>[8x]MGAGAGARWGSRAPEAPQPARAAGPGDVVVPCHGEHQAGIVTPPPSFIALVALDLASTSDRASVERLLRVWTVDIERLTTGRPGLADSEPELALVPAALTVTVGFGPGLLTAAGLRHRAPAWLHPLPPFGIDRLDPAWCDGDVVLQVCADDRTTLAHAVRVLTKEAQGLASVRWVQRGFRRSPGISEPDGTSMRNLMGQVEGTANLDPRTDPDLLWHRDGEPGWLTGGTSMVVRRIAMNLDTWDELSRGAREATIGRTLRTGAPLTGRAEHDEPDLEALDDHGRPVIDLEAHIRRARPTQREETFLRRAYNYDEAPPPGRASDSGLLFVTYQRDVDAQFTPVQRRLDAADLLNEWTFPVGSAVFAVPGGWSAGEYVGQRLLEG

DyP-type peroxidases (DyPs) are heme-containing enzymes known for their ability to degrade dyes through their peroxidase activity. Based on sequence features, the family of DyPs can be dissected into four subfamilies (class A, B, C, and D DyPs), according to the Peroxibase classification. In this paper we identify another type A DyP from the alkaliphilic cellulomonad, Cellulomonas bogoriensis (CboDyP). Except for typical class A sequence features such as a Tat-signal sequence and the presence of a conserved His to interact with the iron in the heme cofactor, the CboDyP sequence has an aberrant sequence in the region where normally a GXXDG motif is found.

The crystal structure of C. bogoriensis dye-decolorizing peroxidase (CboDyp) was determined to 2.4 Å resolution. The model contains eight protein molecules in the asymmetric unit (molecules A–H). Like other enzymes of this class, CboDyp is a homodimer. The monomer has a characteristic Dyp-type peroxidase fold containing two domains with both a ferredoxin-like fold, consisting of two four-stranded antiparallel β-sheets packed against each other. The porphyrin ring of the heme cofactor is buried in a hydrophobic pocket packed between the β-strands of the N-terminal domain and two α-helices. The heme cofactor is ligated by the strictly conserved proximal His292 with a distance of 2.1 Å between Nε of the imidazole ring and the heme iron. The distal face of the porphyrin ring is ligated by Glu201 and Arg307. A glutamate residue at that position is different from all other DyP peroxidases so far known which all contain an aspartate. The extra methyl group positions the oxygens of the carboxylate group at 4.5 and 4.8 Å from the Fe of the cofactor. Hence the dimensions of the distal cavity near the heme-Fe have been reduced.>[3x]MGSSHHHHHHSSGLEVLFQGPHMETAIWIKNSKLPAVLVAAGAFDAAVQALSKQVGVVKLEPLKKYFTNIYEGCRTYIPSTPCELPAQLGYVRAYDDTVSEDQILPYVPGLDVVNEKMNEGYKNFKLNKPDIAIECF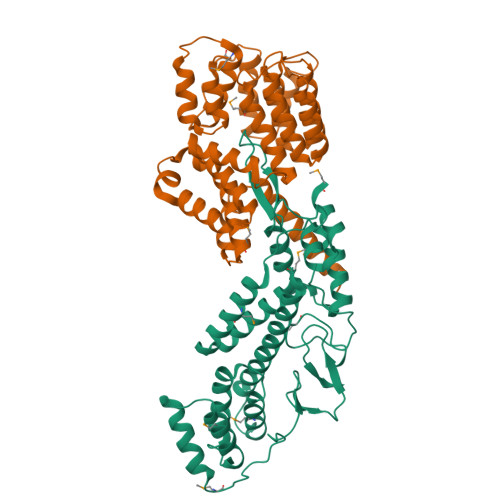REAIYRITLLMVDDAEDEKLAHKILETAREYILGLSIELERRSLKEGNTVRMLELAAYFTKAKLSPIHRTNALQVAMSQHFKHKNFLQASYFAGEFLKIISSGPRAEQARKIKNKADSMASDAIPIDFDPYAKFDICAATYKPIYEDTPSVSDPLTGSKYVITEKDKIDRIAMISKIGAPASGLRIRV;>[3x]MGSSHHHHHHSQDPMDYFNIKQNYYTGNFVQCLQEIEKFSKVTDNTLLFYKAKTLLALGQYQSQDPTSKLGKVLDLYVQFLDTKNIEELENLLKDKQNSPYELYLLATAQAILGDLDKSLETCVEGIDNDEAEGTTELLLLAIEVALLNNNVSTASTIFDNYTNAIEDTVSGDNEMILNLAESYIKFATNKETATSNFYYYEELSQTFPTWKTQLGLLNLHLQQRNIAEAQGIVELLLSDYYSVEQKENAVLYKPTFLANQITLALMQGLDTEDLTNQLVKLDHEHAFIKHHQEIDAKFDELVRKYDTSN> 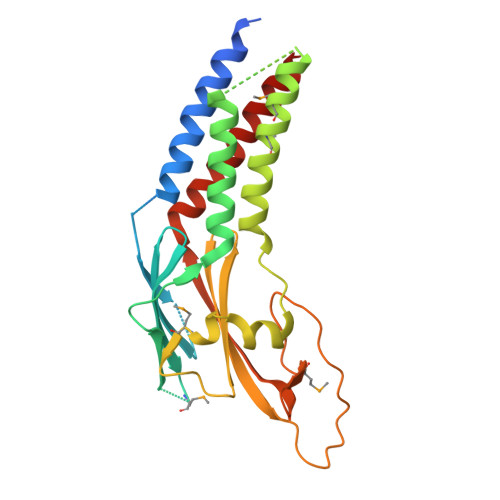SGERAVLEEEFRWLLHDEVHAVLKQLQDILKEASLRFTLPGSGTEGPAKQENFILGSCGTDQVKGVLTLQGDALSQADVNLKMPRNNQLLHFAFREDKQWKLQQIQDARNHVSQAIYLLTSRDQSYQFKTGAEVLKLMDAVMLQLTRARNRLTTPATLTLPEIAASGLTRMFAPALPSDLLVNVYINLNKLCLTVYQLHALQPNSTKNFRPAGGAVLHSPGAMFEWGSQRLEVSHVHKVECVIPWLNDALVYFTVSLQLCQQLKDKIS> MNSSRSVNPRPSFAPRALSLAIALLLGAPAFAANSGEAPKNFGLDVKITGESENDRDLGTAPGGTLNDIGIDLRPWAFGQWGDWSAYFMGQAVAATDTIETDTLQSDTDDGNNSRNDGREPDKSYLAAREFWVDYAGLTAYPGEHLRFGRQRLREDSGQWQDTNIEALNWSFETTLLNAHAGVAQRFSEYRTDLDELAPEDKDRTHVFGDISTQWAPHHRIGVRIHHADDSGHLRRPGEEVDNLDKTYTGQLTWLGIEATGDAYNYRSSMPLNYWASATWLTGDRDNLTTTTVDDRRIATGKQSGDVNAFGVDLGLRWNIDEQWKAGVGYARGSGGGKDGEEQFQQTGLESNRSNFTGTRSRVHRFGEAFRGELSNL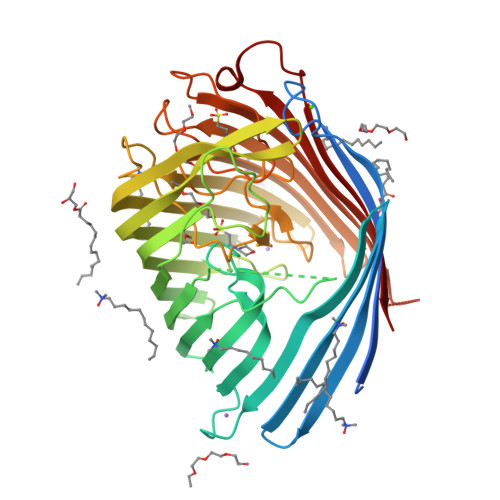QAATLFGSWQLREDYDASLVYHKFWRVDDDSDIGTSGINAALQPGEKDIGQELDLVVTKYFKQGLLPASMSQYVDEPSALIRFRGGLFKPGDAYGPGTDSTMHRAFVDFIWRF> T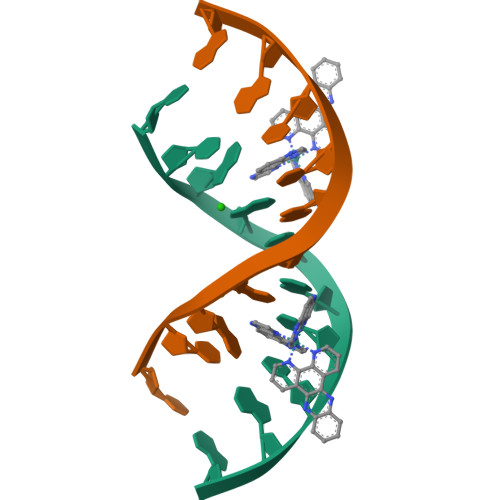CIGCGCCGA>GSHMDASVMSTTYALSAAQTEIWLAQQLYPDSPVYNIAQYTVIEGVIEPAVFEAALRQVIDEADTLRLQFIDSDDGLRQRIGTPAWSMPVLDLTAQADPQAAAQAWMRADYQQPVNLTQGPLFCYALLKVAPAQWMWYQRYHHIMMDGYGAYLIAQRVAYVYSALCEGTTPAECDFGSILQLLESDAQYQISAQRAQDEAYWLKHCANWSEPATLASRSAPVLQQRLRQTTYLAIQALGDTAPDARRLAQFMTAAMAAYLYRFTGEQDVVLGLPVKVRFGADRHIPGMKSNTLPLRLTMRPGMNLSSLMQQAAQEMQSGLRHQRYPSEALRR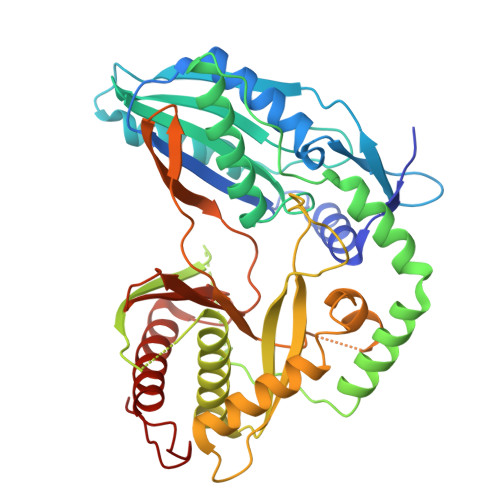QLGMPSGQRLFGTTVNVMPFDLDLSFGGYSATNHNLLNGPAEDLMLGVYWTPGSHQLRIDFDANPACYTPEGLGAHQRRFIRFMQVLAADATQPIDSIDLLD[4x]> MTPQALKIIVPYPAGGTA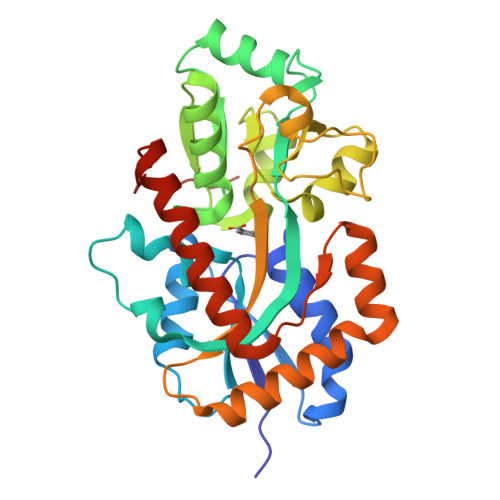DILPRVVAEKLRAQFPAGVLIDNRTGAGGNIGAEAVFRAEPDGNTLLASPPGPIAINHHLYRKMAFDPSKWEPVTVLATVPNVLVVNPRLPVKNVQEFIAYAKANPGKVTYGSQGNGTTSHLTASLFMQLTGTEMVHVPYDGTAPALVDLVGGQIDVFFDNISSSLPFHQAGKLRILGVADEQRSAALPEVPTFAEQGLPSMNAVTWFAVVAPPGTPAAKVAALQKSFAGALTQPEVQQKFAEQGAEPRGWDPARTGQFIRAESAKWDRVIRSANVRLDLEHHHHHH1-[(2R,3aR,4R,6R,6aR)-2-hydroxy-6-(hydroxymethyl)-2-sulfidotetrahydrofuro[3,4-d][1,3,2]dioxaphosphol-4-yl]pyrimidine-2,4(1H,3H)-dione 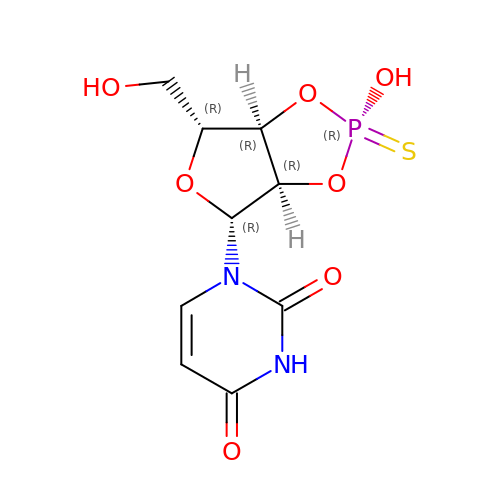| C9 H11 N2 O7 P S | OIDQHQCLWHMGIL-VQAIERIMSA-N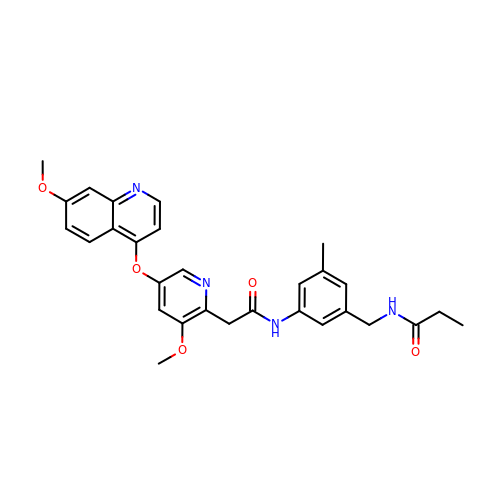~{N}-[[3-[2-[3-methoxy-5-(7-methoxyquinolin-4-yl)oxy-pyridin-2-yl]ethanoylamino]-5-methyl-phenyl]methyl]propanamide | C29 H30 N4 O5 | MXZGKLMWAXAYIG-UHFFFAOYSA-N> G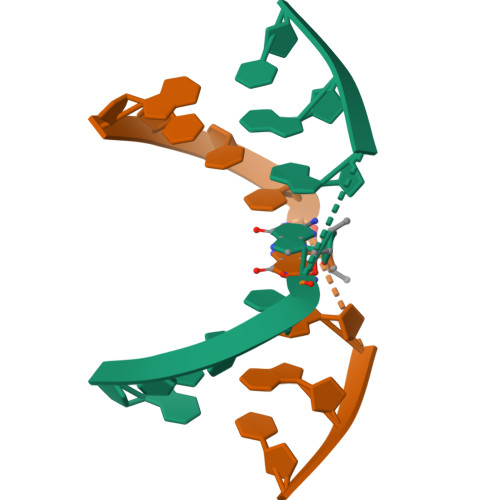CCCGGGC> MTSLFEPAQAGDIALANRIVMAPLTRNRSPGAIPNNLNATYYEQRATAGLIVTEGTPISQQGQGYADVPGLYKREAIEGWKKITDGVHSAGGKIVAQIWHVGRISHTSLQPHGGQPVAPSAITAKSKTYIINDDGTGAFAETSEPRALTIDDIGLILEDYRSGARAALEAGFDGVEIHAANGYLIEQFLKSSTNQRTDDYGGSIENRARFLLEVVDAVAEEIGAGRTGIRLSPVTPANDIFEADPQPLYNYVVEQLGKRNLAFIHVVEGATGGPRDFKQGDKPFDYASFKAAYRNAGGKGLWIANNGYDRQSAIEAVESGKVDAVAFGKAFIANPDL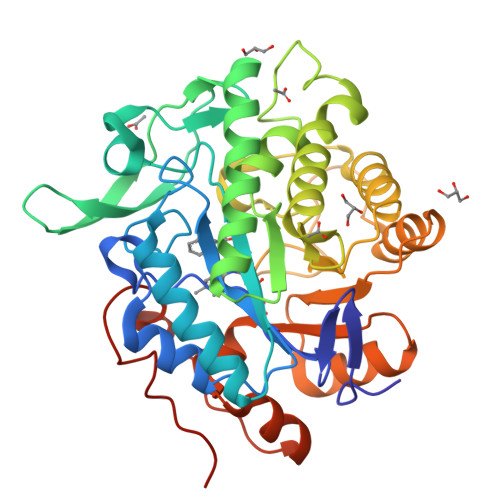VRRLKNDAPLNAPNQPTFYGGGAEGYTDYPALAQLEHHHHHH> MAFSELLDLVGGLGRFQVLQTMALMVSIMWLCTQSMLENFSAAVPSHRCWAPLLDNSTAQASILGSLSPEALLAISIPPGPNQRPHQCRRFRQPQWQLLDPNATATSWSEADTEPCVDGWVYDRSIFTSTIVAKWNLVCDSHALKPMAQSIYLAGILVGAAACGPASDRFGRRLVLTWSYLQMAVMGTAAAFAPAFPVYCLFRFLLAFAVAGVMMNTGTLLMEWTAARARPLVMTLNSLGFSFGHGLTAAVAYGVRDWTLLQLVVSVPFFLCFLYSWWLAESARWLLTTGRLDWGLQELWRVAAINGKGAVQDTLTPEVLLSAMREELSMGQPPASLGTLLRMPGLRFRTCISTLCWFAFGFTFFGLALDLQALGSNIFLLQMFIGVVDIPAKMGALLLLSHLGRRPTLAASLLLAGLCILANTLVPHEMGALRSALAVLGLGGVGAAFTCITIYSSELFPTVLRMTAVGLGQMAARG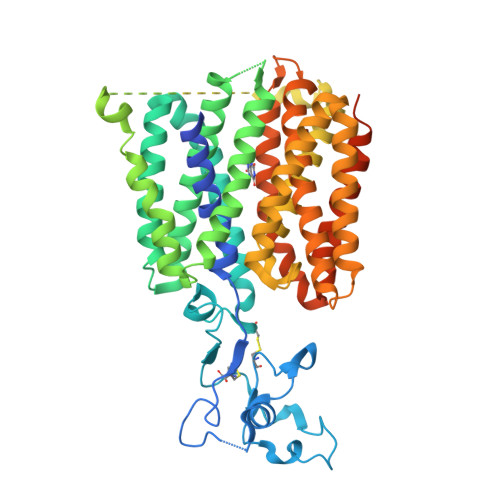GAILGPLVRLLGVHGPWLPLLVYGTVPVLSGLAALLLPETQSLPLPDTIQDVQNQAVKKATHGTLGNSVLKSTQF>MRGSHHHHHHGLVPRGSMIRTMLQGKLHRVKVTHADLHYEG[2x];>CCAIDQDFLDAAGILENEAIDIWNVTNGKRFSTYAIAAERGSRIISVNGAAAHCASVGDIVIIASFVTMPDEEARTWRPNVAY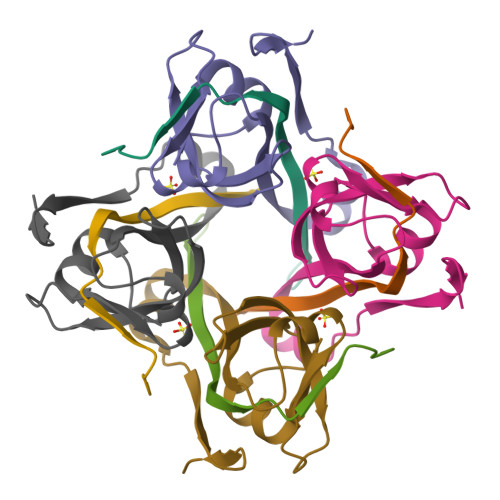FEGDNEMKRTAKAIPVQVA[2x]>FADDHAMSPDMKLLAGASNWVNQSGSVAQFVFTPSPTQPQTYEVSGNYINNAQGTGCKGTPYPLSGAYYSGNQIISFSVVWSNASANCQSATGWTGYFDFSGSQAVLKTDWNLAFYSGSTPAIQQGQDDFMQSV[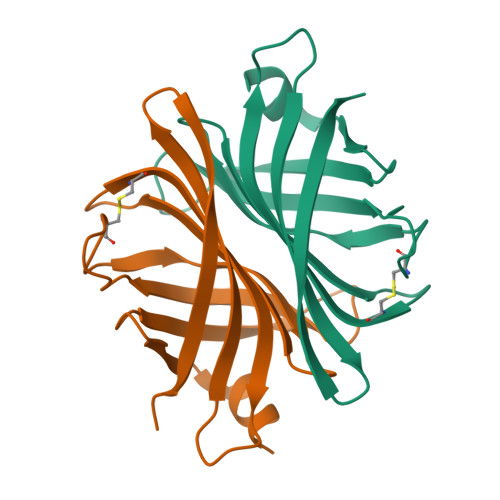2x]> GSHMEELQNKLEDVVIDRNLLILGRILGEGEFGSVMEGNLKQEDGTSLKVAVKTMKLDNSSQREIEEFLSEAACMKDFSHPNVIRLLGVCIEMSSQGIPKPMVILPFMKYGDLHTYLLYSRLETGPRHIPLQTLLRFMVDIALGMEYLSNRNFLHRDLAARNCMLRDDMTVCVADFG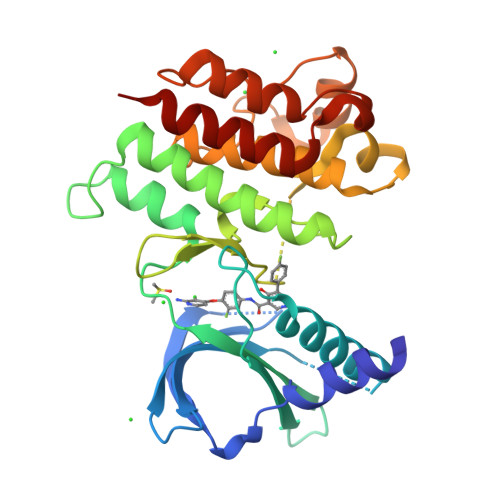LSKKIYSGDYYRQGRIAKMPVKWIAIESLADRVYTSKSDVWAFGVTMWEIATRGMTPYPGVQNHEMYDYLLHGHRLKQPEDCLDELYEIMYSCWRTDPLDRPTFSVLRLQLERLLESLPDV>[2x]MHHHHHHENLYFQGHMAPDELASLEKDFGGRIGVYALDTGSGDTVGHRADERFLMCSTVKTFIVSAILRRRLSEPGLLDQRIQYTQSDVLEWAPITSQHV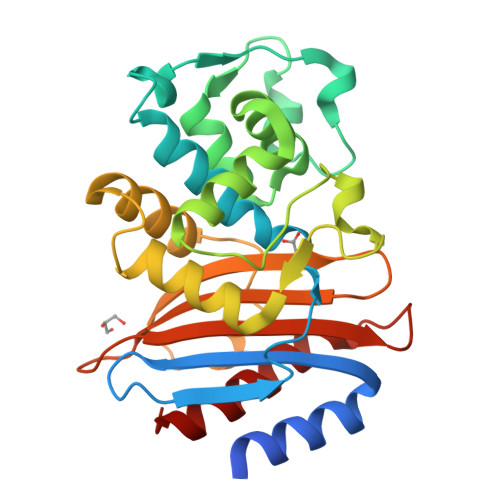STGMTVSELCDATLRYSDNTGANLLITQLGGPKETEKFVRSLGDNVTRMDRTEVQLNIPDGDLDTSTPQQLVANLRRLVLDEGLDSRGRDLLTDWLKRNTTGDQSIRAAVPAGWTVADKTGGGFKGETNDIAVIWPPGRAPIVMAVLTVPEDPTSTKGKPTIAAATRIVLRAFGA5-amino-1-tert-butyl-3-(quinolin-2-yl)-1H-pyrazole-4-carboxamide 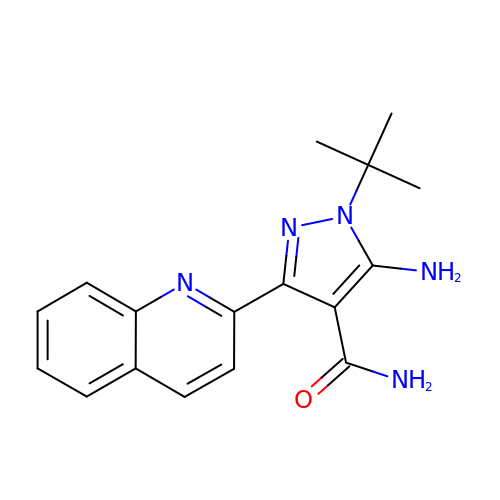| C17 H19 N5 O | YKVANMRHVMVLJX-UHFFFAOYSA-N>[2x]GSGSAMIEARQVSELSTRIISSVQMLSNAQNEQERKEAGRVLFEQLESLLTHIKELGGESFDSKLLDALESNVQNVINNLAELGVTVERKLWLAKEIDTRVEEMRLLSEELEQLTRTQVQNTSTIAVANVTHIYDLLEANKKDQVYQALDALVEVDLDLTERLHELHLLAFKMLNQIEEARTLTNVDRIQQIQTAFE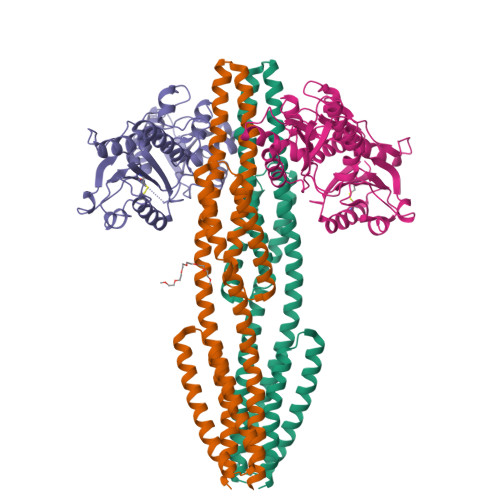NNLKIMKRRVLAVEDPTRSKQMSQLLTELGKRQVVFTILLQQYENNEQSQQLMQKTLELFSELNSTVNKLVDDSNKTTTK;>[2x]GSGSDEKICAIYPHLKDSYWLSVNYGMVSEAEKQGVNLRVLEAGGYPNKSRQEQQLALCTQWGANAIILGTVDPHAYEHNLKSWVGNTPVFATVNQLDLDEEQSTLLKGEVGVDWYWMGYEAGKYLAERHPKGSGKTNIALLLGPRTRGGTKPVTTGFYEAIKNSDIHIVDSFWADNDKELQRNLVQRVIDMGNIDYIVGSAVAIEAAISELRSADKTHDIGLVSVYLSHGVYRGLLRNKVLFAPTDKMVQQGRLSVMQAAHYLRHQPYEKQASPIIKPLTPKTLHDDTIEESLSPSEYRPTFS>EQLSFDELTLINLSKVVTVNGHEVPMRIKEFELLWYLASRENEVISKSELLEKVWGYDYYED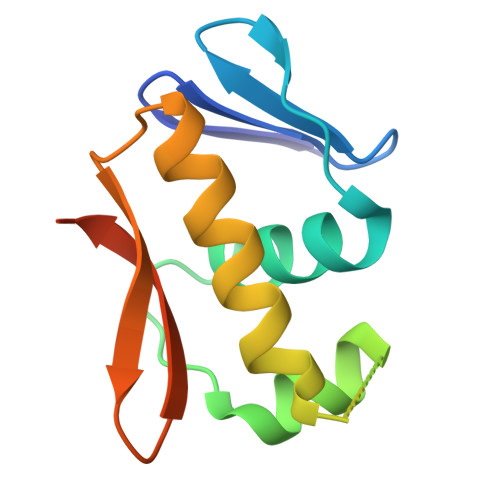ANTVNVHIHRIREKLEKESFTTYTITTVWGLGYKFERSRLEHHHHHH[2x]>MSDKDSKNTPQVPEKLGLSRRGFLGASAVTGAAVAATALGGAVMTRESWAQAVKESKQKIHVGPGELDDYYGFWSGGHQGEVRVLGVPSMRELMRIPVFNVDSATGWGLTNESRHIMGDSAKFLNGDCHHPHISMTDGKYDGKYLFINDKANSRVARIRLDIMKCDKMITVPNVQAIHGLRLQKVPHTKYVFANAEFIIPHPNDGKVFDLQDENSYTMYNAIDAETMEMAFQVIVDGNLDNTDADYTGRFAAATCYNSEKAFDLGGMMRNERDWVVVFDIHAVEAAVKAGDFITLGDSKTPVLDGRKKDGKDSKFTRYVPVPKNPHGCNTSSDGKYFIAAGKLSPTCSMIAIDKLPDLFAGKLADPRDVIVGEPELGLGPLHTTFDGRGNAYTTLFIDSQVVKWNMEEAVRAYKGEKVNYIKQKLDVHYQPGHLHASLCETNEADGKWLVALSKFSKDRFLPVGPLHPENDQLIDISGDEMKLVHDGPTFAEPHDCIMARRDQIKTKKIWDRNDPFFAPTVEMAKKDGINLDTDNKVIRDGNKVRVYMTSMAPAFGVQEFTVKQGDEVTVTIT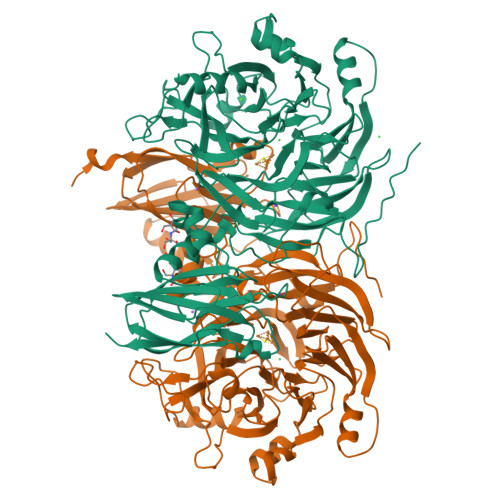NIDQIEDVSHGFVVVNHGVSMEISPQQTSSITFVADKPGLHWYYCSWFCHALHMEMVGRMMVEPAWSHPQFEK[2x]> MLDRFATKQTQEKLKIGVVGVFAIGCLFPLLSDFKRSYPHIDLHISTHNNRVDPAAEGLDYTIRYGGGAWHDTDAQYLCSALMSPLCSPTLASQIQTPADILKFPLLRSYRRDEWALWMQTVGEAPPSPTHNVMVFDSAVTMLEAAQAGMGVAIAPVRMFTHLLSSER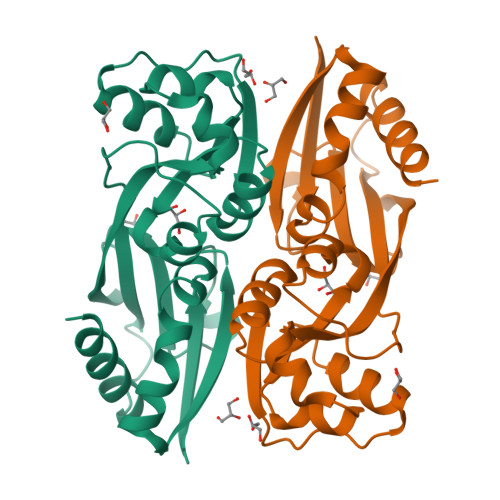IVQPFLTQIDLGSFWITRLQSRPETPAMREFSRWLTGVLHKTSGSHHHHHH> GSPDETDGFVKQKSERVYHLDFNQTPTGVTLNNGVTAFPYYEHGNDANVQS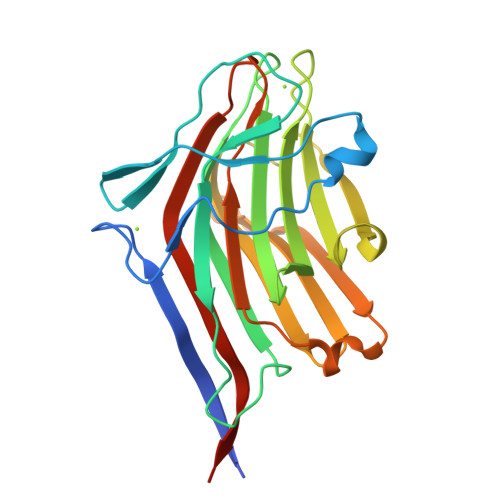GPFGYANGIAYPSTERTASNYWNGPSMSGTIPKNSNGSNTANFQFVNRVNVGTNAAEVGRFEFNLTYQGKIVASLALFDDSASNDQWVFSGTVYDGSQAQMLFFDLLPRNYYRDGNYNAVITKMGDQLTFRLDRIDLGDGGIETRTVSGFSSVPIDGWTAWFPGFSDQRGWSINWQDSYFEWINVDYWDDIPNRFK Bilin 584 (single linked) | C33 H38 N4 O6 | 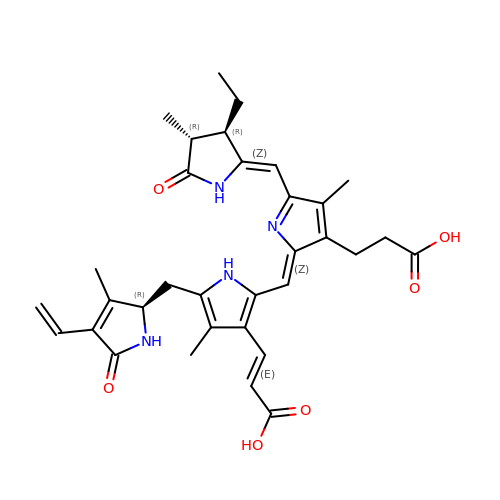DELSVXYVYXKOJW-GUEBWASOSA-N5-(pyridin-2-yl)thiophene-2-carbothioamide 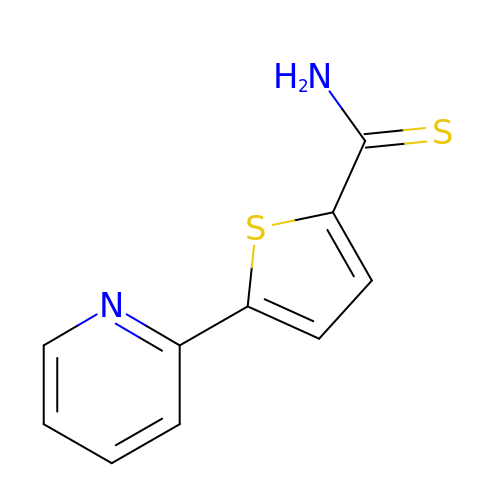| C10 H8 N2 S2 | VOYHCOULKKDLRP-UHFFFAOYSA-N> GSMNQATQIIPFTTSGSLVDYVDRKVIVVLRDGKKLIGILRSFDQFANLMLQYTIERIYVDDMYGDIDRGVYIVRGENVVLLGELD;> MLFYSFFKTLIDTEVTVELKNDMSIRGILKSVDQFLNVKLENISVVDASKYPHMAAVKDLFIRGSVVRYVHMSSAYVDTILLADACRRDLANNKRQ;> GSMESAQAVAEPLDLVRLSLDEIVYVKLRGDRELNGRLHAYDEHLNMVLGDAEEIVTIFDDEET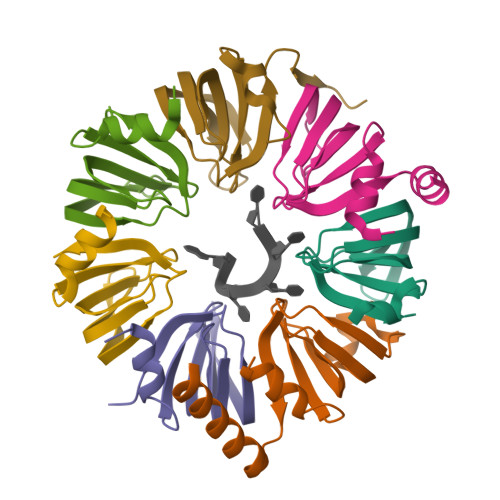DKDKALKTIRKHYEMLFVRGDSVILIAPPRN;> MLPLTLLNATQGRPILVELKNGETFNGHLENCDNYMNLTLREVIRTMPDGDKFFRLPECYIRGNNIKYLRIQDEVLSQVAKQQAQQRENRGSRFRGRGQRGRGNYGHTAPNRRGRGRGGHMWSHPQFEK;> MSMTILPLELIDKCIGSNLWVIMKSEREFAGTLVGFDDYVNIVLKDVTEYDTVTGVTEKHSEMLLNGNGMCMLIPGGKPE;> GSMDSSPNEFLNKVIGKKVLIRLSSGVDYKGILSCLDGYMNLALERTEEYVNGKKTNVYGDAFIRGNNVLYVSALDD;> MSSLQKRPGPGNSSQPTERPRKESILDLSRYQDQRIQATFTGGRQITGILKGFDQLMNLVLDDVEEQLRNPEDGKLTGAIRKLGLVVVRGTTLVLIAPMDGSEEIPNPFVQAEHHHHHH> TTPLVHVASVEKGRSYEDFQKVYNAIALKLREDDEYDNYIGYGPVLVRLAWHTSGTWDKHDNTGGSYGGTYRFK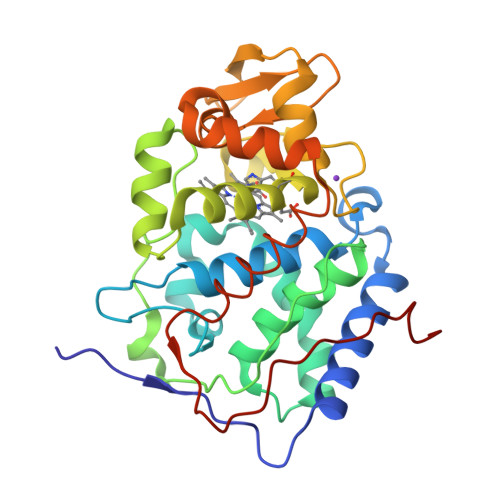KEFNDPSNAGLQNGFKFLEPIHKEFPWISSGDLFSLGGVTAVQEMQGPKIPWRCGRVDTPEDTTPDNGRLPDADKDADYVRTFFQRLNMNDREVVALMGAHTLGKTHLKNSGYEGPWTANNNVFDNSFYLNLLNEDWKLEKNDANNEQWDSKSGYLQLPTDYSLIQDPKYLSIVKEYANDQDKFFKDFSKAFEKLLENGITFPKDAPSPFIFKTLEEQGL> MGSSHHHHHHSQDPKPRVLVLTGAGISAESGIRTFRAADGLWEEHRVEDVGTPEGFDRDPELVQAFYNARRRQLQQPEIQPNAAHLALAKLQDALGDRFLL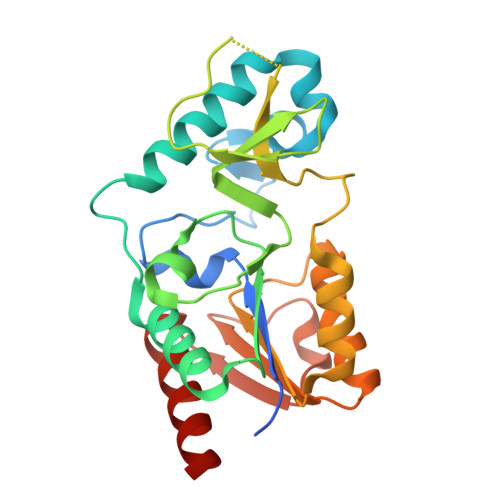VTQNCDNLHERAGNTNVIHMHGELLKVRCSQSGQALDWTGDVTPEDKCHCCQFPAPLRPHVVWFGEMPLGMDEIYMALSMADIFIAIGTSGHVYPAAGFVHEAKLHGAHTVELNLEPSQVGNEFAEKYYGPASQVVPEFVEKLLKGLKAGSIA Secretory-pathway Ca2+-ATPases (SPCAs) play critical roles in maintaining Ca2+ homeostasis, but the exact mechanism of SPCAs-mediated Ca2+ transport remains unclear. Here, we determined six cryo-electron microscopy (cryo-EM) structures of human SPCA1 (hSPCA1) in a series of intermediate states, revealing a near-complete conformational cycle. The overall structure of hSPCA1 is typical of a P-type ATPase, with ten transmembrane (TM) helices (TM1–TM10) and three conserved cytosolic domains: the actuator (A), phosphorylation (P), and nucleotide-binding (N) domains. Structural analysis revealed that the Ca2+ coordinates with the side-chain oxygen atoms of several residues, including Glu308, Asn738, and Asp742, and the main-chain carbonyl oxygen atoms of other residues, including Val303, Ala304, and Ile306, consistent with the results reported by Chen et al. We also found that the Ca2+-binding site in hSPCA1 corresponds to site II in hSERCA2.

To gain insight into how hSPCA1 recognizes Ca2+, we successfully obtained the structures of hSPCA1 bound to Ca2+ in three different states: CaE1, CaE1-ATP, and CaE1P-ADP. We found that the TMDs were nearly identical in all three structures. In hSPCA1, the N domain interacted with the P domain through several residues, including Gly518, Ser519, Ala520, Gly521, Ile545, Glu575, Thr576, Ala579, and Ile580, with a distance between the 480KGA motif and the 350DKT motif at ~25.0 Å. Meanwhile, the A domain interacted with the P domain through multiple residues, including Val165, Gly166, Asp167, Arg168, and Leu222 in the A domain, and Val646, Asp667, Val668, and Glu671 in the P domain, with a distance of 33.2 Å from the 350DKT motif to the 189TGE motif. As expected, there was no interaction observed between the A and N domains. No significant conformational changes were observed in the TMD and the A and P domains during the transition of CaE1 → CaE1-ATP, with the root mean square deviation (RMSD) being 0.83 Å. MD simulations of the CaE1 state showed a solvent-accessible cavity facing the cytosol formed by TM1, TM2, and TM4. This cavity provided access to the Ca2+-binding site, suggesting a possible entry pathway for Ca2+. During the Ca2+ transport cycle, hSPCA1 starts with a loosely arranged headpiece of cytosolic domains, with the N domain ready to bind ATP. Ca2+ from the cytosol can then enter the binding site through the cytosol-facing cavity.

> MKVARFQKIPNGENETMIPVLTSKKASELPVSEVASILQADLQNGLNKCEVSHRRAFHGWNEFDISEDEPLWKKYISQFKNPLIMLLLASAVISVLMHQFDDAVSITVAILIVVTVAFVQEYRSEKSLEELSKLVPPECHCVREGKLEHTLARDLVPGDTVCLSVGDRVPADLRLFEAVDLSIDESSLTGETTPCSKVTAPQPAATNGDLASRSNIAFMGTLVRCGKAKGVVIGTGENSEFGEVFKMMQAEEAPKTPLQKSMDLLGKQLSFYSFGIIGIIMLVGWLLGKDILEMFTISVSLAVAAIPEGLPIVVTVTLALGVMRMVKKRAIVKKLPIVETLGCCNVICSDKTGTLTKNEMTVTHIFTSDGLHAEVTGVGYNQFGEVIVDGDVVHGFYNPAVSRIVEAGCVCNDAVIRNNTLMGKPTEGALIALAMKMGLDGLQQDYIRKAEYPFSSEQKWMAVKCVHRTQQDRPEICFMKGAYEQVIKYCTTYQSKGQTLTLTQQQRDVYQQEKARMGSAGLRVLALASGPELGQLTFLGLVGIIDPPRTGVKEAVTTLIASGVSIKMITGDSQETAVAIASRLGLYSKTSQSVSGEEIDAMDVQQLSQIVPKVAVFYRASPRHKMKIIKSLQKNGSVVAMTGDGVNDAVALKAADIGVAMGQTGTDVCKEAADMILVDDDFQTIMSAIEEGKGIYNNIKNFVRFQLSTSIAALTLISLATLMNFPNPLNAMQILWINIIMDGPPAQSLGVEPVDKDVIRKPPRNWKDSILTKNLILKILVSSIIIVCGTLFVFWRELRDNVITPRDTTMTFTCFVFFDMFNALSSRSQTKSVFEIGLCSNRMFCYAVLGSIMGQLLVIYFPPLQKVFQTESLSILDLLFLLGLTSSVCIVAEIIKKVERSREKIQKHVSSTSSSFLEV>GAMDDSSLQKVELQTDVYMVCLQHALSTENFEVMGLLIGNFACGIAKISAVIILRRLDKKKDRVEISSEQLLKAAAEAERLTVELNRPMRVLGWYQSQPHITVCPSHVDVRTQATYQTMDHSFVGLIFSVFSEGKESKEHEIFLNCFQSDNGEATEIPLEIVHTPDISDRCLRTMTDLSKILVQEEEDMAEACKDHPDVLASIHNNAVRTRALIHITDIITKPLVQTFEKRIALNKLRATHLQRQLQELQKMCNG[2x];>[2x]MADSDLLVTISGAALSLLFFENVRSVGNQMGFLLGEALEFIVKTYTDSDNQVETVKIHINVEAIVTCPLADLLHDSTNHINKEKLKDFVRDKSKQVIGWFCFRRNTTNLTLTLKDKLLHKQFASHFSGVNGCKEDFFLTCLLNASTSETSGTHKFRHVFLRHNKRGMFEPISLKINNLGDDASRHDGSDYKPTPVRKSTRTPDSFTKLIESLNLDVARIDGLDSAMLIQKAAEHHLMSLIPKVCESDLEVAELEKQVHELK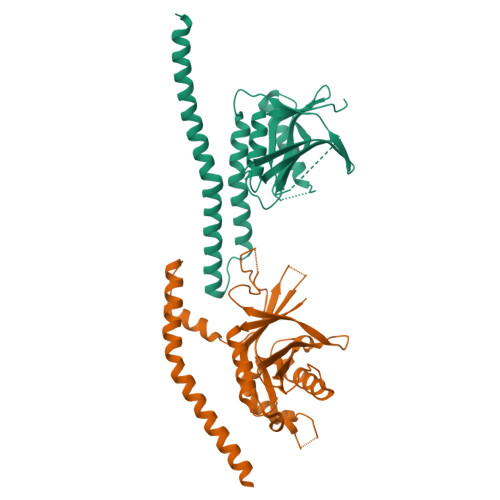IKIATQQLAKRLKINGENCDRISKASKD>MSLENKENLVVIDLAIAEDSIQKKNIVYDKNGQNHFDVISAFIKSIRGSDPDATLYWLANMVEAGEDPNFIFRRLLISACEDIGLADPNAIVVVQSCCDAFDRVGFPEGLFFLSQASLYLAISPKSNSTKSIFKAMEAIKATNVSLVPNHLKNNASNYLNPHNYQGKWL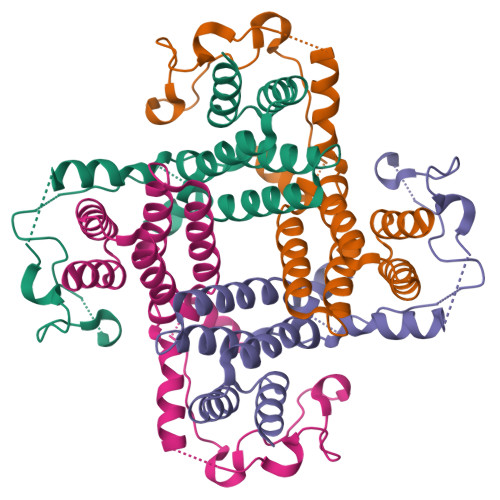QQEYLPTDLQGIKFWKPKDSGWEKNKYEDLPKKQKSEGHHHHHH[2x]>[2x]SNAMRASLKASLAGAALLLAAAVAPAAQAGPDQQFFPLATYR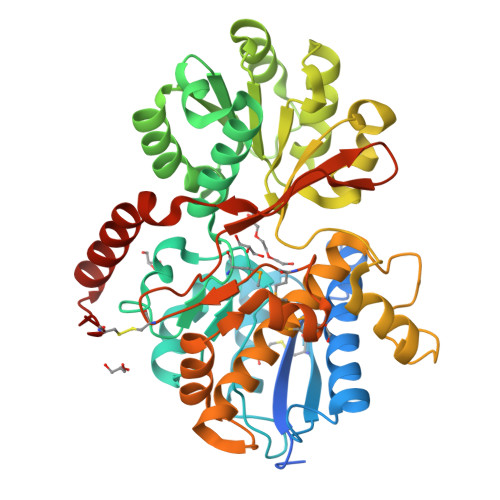VGAYASSGVQVWAGMIDYLNYINQVEGGINGVKLVWQECETEWTAEKGIECYERFKNGLDGAPVAVYQPNGAPAAYALSERAEVDKIPLITLGYGRTEATDGTVFPYNFPVMLTFYSEASTLVNYIAQREGGFDRLKGKKIATLYHDSAYGRETLGPLKLLAEKYGFENIQIPVADPGNEQSAQWRQIRQQNPDWVFLRTWGVSTPVAVKTAARFGFPVDHIIGDIWASSSEDVLPAGAAAKGYLALTPYPAGSDFEIHKRLKQYILDTGKSDLKDLKNFGSVYYNSGLVNAAVAVEAIRTAQGKFGKRPLNGEEGRWGLEHLNIDDARLKDMGYLGLMQNLKLSCRDHEGGGAARVQQWDGANWTLISEWIAADRALLRPLIDEKAAAFAKEKRLVPRTCNEGD>HHHHASILIDTSAWVEYFRATGSIAAVEVRRLLSEEAARIAMCEPIAMEILSGALDDNTHTTLERLVNGLPSLNVDDAIDFRAAAGIYRAARRAGETVRSINDCLIAALAIRHGARIVHRDADFDVIARITNLQAASFR[4x];>SRTNIDIDDELAAEVMRRFGLTTKRAAVDLALRRLVGSPLSREFLLGLEGVGWEGDLDDLRS[4x]

Virulence-associated proteins B and C (VapBC) are the most abundant Type II TA system present in prokaryotes. VapC, the toxin, inhibits protein translation by cleaving either transfer RNA (tRNA) or the sarcin-ricin loop (SRL) of 23S ribosomal RNA (rRNA) or messenger RNA (mRNA), and this activity is neutralized by their cognate VapB antitoxins. Here, we demonstrate that the VapBC11 TA module is essential for Mtb to establish infection in guinea pigs. In the present study, we also show that VapC11 cleaves tRNA-LeuCAG in a Mg2+-dependent manner.

The VapBC11 complex crystallized in the P212121 space group, and the structure was solved at 1.67 Å resolution using molecular replacement, as described in the ‘Materials and Methods’ section. The asymmetric unit consisted of four chains each of VapB11 and VapC11. VapB11 and VapC11 interact to form a VapB4C411 heterooctameric complex. As expected, VapC11 adopts canonical PIN domain fold architecture β(1)α(6)β(1)α(1)β(1) topology. The N-terminal domain (∼1–40 amino acids) in VapB11 forms a RHH structural motif. We observed that the α3 helix docks at the lateral site, while α4 interacts with the active site residues of VapC11. Consequently, this mode of interaction may sterically occlude the tRNA-binding site of the toxin. The overall architecture of VapBC11 adopts a closed conformation, where two VapC11 homodimers additionally interact at the α4 and α5 of diagonally positioned VapC chains. The highly conserved Arg (i.e. Arg62) in VapB11 forms complex salt bridge interactions with highly conserved active site residues Asp5, Glu44 and Asp116 of VapC11. These interactions consequently overlap with the potential metal ion binding site of VapC11.Bacterial HSS is mostly found in α-proteobacteria and in some β- and γ-proteobacteria, including pathogenic strains such as Legionella pneumophila, Brucella spp. and various P. aeruginosa strains, including PA7 and PA14. It catalyzes the conversion of two molecules of putrescine (PUT; 1,4-diaminobutane) into one molecule of sym-homospermidine [HSP; bis(4-aminobutyl)amine] as the main reaction along with several side reactions (Ober et al., 1996; Böttcher et al., 1994). Bacterial HSS is NAD+-dependent, active at neutral to basic pH with an optimum at pH ∼8.8, and shows increased activity in the presence of 50 mM potassium ion. BvHSS forms a dimer, with each subunit containing a boot-shaped substrate-binding pocket between an NAD(P)-binding Rossmann-like domain and an HSS-like domain. The cofactor NAD+ is bound as a prosthetic group in the binding pocket with its nicotinamide ring being part of the active site.

An ‘ionic slide’ (residues Asp94 and Glu117) was proposed to lead positively charged amine substrates from the entrance to the binding pocket into the active site. The activity of these BvHSS variants in relation to wild-type BvHSS correlated to the negative electrostatic potential of the exchanged residue in the order D94N (61%) > D94K (52%) >>> E117Q (1.5%) > E117K (inactive). The deeper lying residue Glu117 consistently had far more influence on the activity than Asp94 at the pore opening. Due to a lack of interpretable electron density, large parts of the ‘track-and-trace’ loops are missing in the BvHSS variant E117Q (residues 123–127 are missing in chain A and residues 121–127 in chain B). The shifted side chain of Gln117 is thereby moved away from the entrance tunnel and does not cause steric occlusion. In addition, the electron-density distribution of the NAD+ molecule was interpreted as alternative ribose conformers of the nicotinamide riboside moiety. While the ribose moiety in the wild-type structure is exclusively present as a C2′-endo conformer, both C2′-endo and C3′-endo conformers seem to be present in the BvHSS variant E117Q. However, the extent of the above-described structural deviations is rather small and should not exert significant effects on the activity of the variant. Instead, the drastically reduced activity of the BvHSS variant E117Q is assumed to be caused by the lack of negative charge at position 117.

>GPMGTDWPVYHRIDGPIVMIGFGSIGRGTLPLIERHFAFDRSKLVVIDPSDEARKLAEARGVRFIQQAVTRDNYRELLVPLLTAGPGQGFCVNLSVDTSSLDIMELARENGALYIDTVVQPWLGFYFDPDLKPEARSNYALRETVLAARRNKPGGTTAVSCCGANPGMVSWFVKQALVNLAADLGVTGEEPTTREEWARLAMDLGVKGIHIAERDTQRASFPKPFDVFVNTWSVEGFVSEGLQPAELGWGTFERWMPDNARGHDSGCGAGIYLLQPGANTRVRSWTPTAMAQYGFLVTHNESISIADFLTVRDAAGQAVYRPTCHYAYHPCNDAVLSLHEMFGSGKRQSDWRILDETEIVDGIDELGVLLYGHGKNAYWYGSQLSIEETRRIAPDQNATGLQVSSAVLAGMVWALENPNAGIVEADDLDFRRCLEVQTPYLGPVVGVYTDWTPLAGRPGLFPEDIDTSDPWQFRNVLVRD[2x]>[2x]MSSPASWNKEDFPWSGKVKDVLQNVFKLQKFRPLQLETINVTMSGKEVFLVMPTGGGKSLCYQLPALCSDGFTLVICPLISLMEDQLMVLKQLGISATMLNASSPKEHVKWVHAEMVNKNSKLKLIYVTPEKIAKSKMFMSRLEKAYEARRFTRIAVDEVHCCSQWGHDFRPDYKALGILKRQFPNASLIGLTATATSHVLKDAQKILCVEKCFTFTASFNRPNLYYEVRQKPSN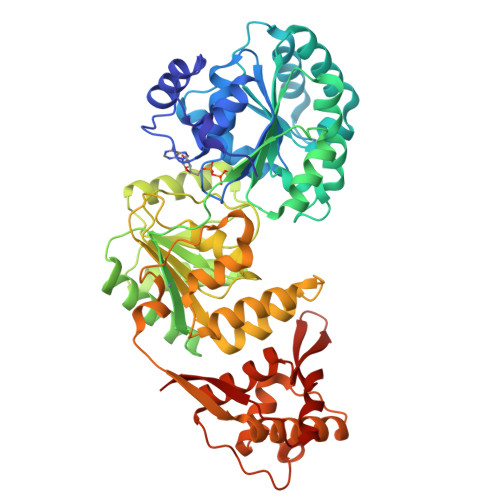TEDFIEDIVKLINGRYKGQSGIIYCFSQKDSEQVTISLQKLGIPAGAYHANMEPEDKTKVHRRWAANEIQVVVATVAFGMGIDKPDVRFVIHHSMSKSMENYYQESGRAGRDDMKADCILYYGFGDIFRISSMVVMENVGQQKLYEMVSYCQNINKCRRVLIAQHFDEVWSPEACNKMCDNCCKEISFERKNVTAYCRDLIKILKQAEDLNEKLTPLKLIDSWMGKGASKLRVAGLAPPTLPREDLEKIIAHFLIQQYLKEDYSFTAYATISYLKVGPKANLLNNEAHVITMRVKK> GSAMGSSSVAISKPLLKLKLLDALRQGSFPNLQDLLKKQFQPLDDPNVQQVLHLMLHYAVQVAPMAVIKEIVHHWVSTTNTTFLNIHLDL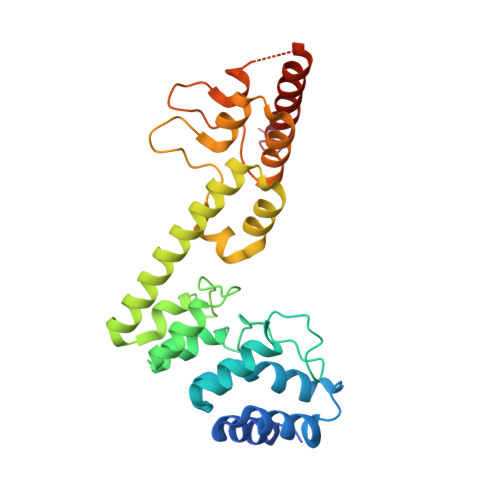NERDSNGNTPLHIAAYQSRGDIVAFLLDQPTINDCVLNNSHLQAIEMCKNLNIAQMMQVKRSTYVAETAQEFRTAFNNRDFGHLESILSSPRNAELLDINGMDPETGDTVLHEFVKKRDVIMCRWLLEHGADPFKRDRKGKLPIELVRKVNENDTATNTKIAIDIELKKLLERATREQSVIDVT>SNAMSLEMFDKEIFDLTNKELERQCEGLEMIASENFTLPEVMEVMGSILTNKYAEGYPGKRYYGGCEFVDEIETLAIERCKKLFNCKFANVQPNSGSQANQGVYAALINPGDKILGMDLSHGGHLTHGAKVSSSGKMYESCFYGVELDGRIDYEKVREIAKKEKPKLIVCGASAYARVIDFAKFREIADEIGAYLFADIAHIAGLVVAGEHPSPFPYAHVVSSTTHKTLRGPRGGIIMTNDEELAKKINSAIFPGIQGGPLMHVIAAKAVGFKFNLS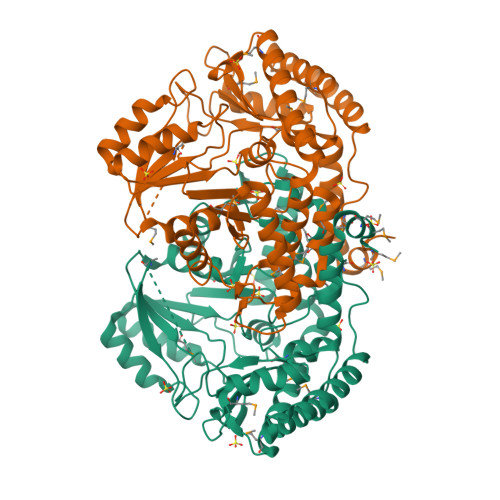DEWKVYAKQVRTNAQVLANVLMDRKFKLVSDGTDNHLVLMSFLDREFSGKDADLALGNAGITANKNTVPGEIRSPFITSGLRLGTPALTARGFKEKEMEIVSNYIADILDDVNNEKLQENIKQELKKLASNFIIYERAMF[2x]> MPSYLSPGVYVEEVASGSRPIEGVGTSVAAFVGLAPTGPL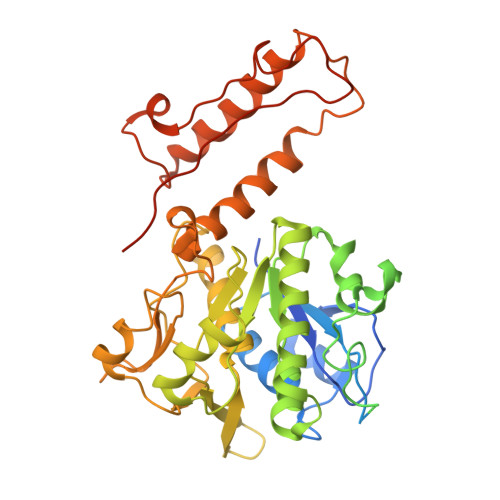NEPTLVTNWTQYVAAFGDFTGGYYLAHSVYGFFNNGGSAAYVVRVGGSAEDAAADGSVNGAAAPAAVTGSTAKALPAAEPKQLGTFAVTATAAGQSGPLTVEVADPEGEGPAERFKLIVKDGDKPVETFDVSAKKGNRSYVVTQVKERSKLITVTEAAPSAQLVRPENQSLTLPAPPSAAPAVPAGQAESAHPGPAQYLGDSSDRTGFGGLEAIDEISMVAVPDLMAAYQRGAIDLEAVKAVQLGLIAHCELMGDRVAIIDPPPNQNARQIRVWRQETAGYDSKYAALYYPWIKSFDPATGQSRLVPPSGHVAGIWARNDSERGVHKAPANEVVRGAVDLELQITRGEQDLLNPIGVNCIRSFPGRGIRVWGARTLSSDPAWRYLNIRRYFNYLEESILIGTQWVVFEPNDHNLWARIRRNVSAFLVNEWRNGALFGQSPDQAYYVKCDEETNPPESVDLGRVVCEIGIAPVKPAEFVIFRLAQFSSGGGELDE>MSKKRVVKLRELVPAVAALAVAVLIQSATGSSGGSGHTPTTQATHADDHDLTTHNGTEEHDDGHDDGHDDLHAHAPKVIVFISGSCLFGAISRSLFKKLPIPYTVVLLILGAILGVVASNVPLVEEHTRDVAHMDPHVLLQIFLPVLIFESAFAMDVHTFMRSFSQVCILALFGLVVASVLTAVLAMNLFNYNWNFSEAMMFGAIMSATDPVAVVALLKDLGASKQLGTIIEGESLLNDGCAIVIFNVFMKMVFFPQLTSTVGQNVLYFLQVAVAGPLWGYAVAKVTVFFLSHIFNDALVEITITLAATYLTYYIGDIWLEVSGVLAVVVLGLIVNAEKTSISPEVEVFLHRFWEMLAYLANTLIFMMVGVVVTQKALVAVDKMDWFYLIILYLAIT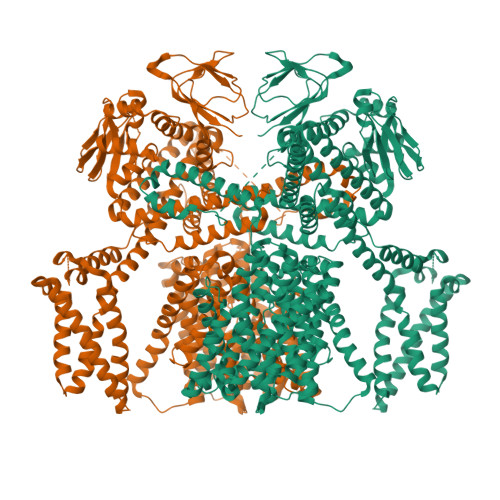IIRGMVISLFSPILSRIGYGLTWRNAVIMTWGGLRGAVGLALALVVENLAGNDVIGSKFLFHTAGIVVLTLVINATTIQTLLRILGMSDISIPKRLAMAGAVRRIHEGQNRTLNMLKSDRFLADADWDIATAACEISDPYSALSDDENAPADELTLGERKSVCPGCKAMVPNEPSPREFADMMEEARLRMLKAEKISYWKQFEHGMLAREALRLLVQHAEVAADEKDQFILVDDLKKSWQIKGIYPWLKRKLEDLISEKKIAAIPMPKYKLGKLMYKICHHMAFEVTINIAIVLNIVPIIMEFVVQDKMASVSTMAAPGSTVSSEPSSLQKIEDALRISNYVFFVIYAIEAIVKILGLGRHYIVSHWNKFDAFILVVALVDIIIAETLLKGSITINLSSIKVVKLFRLLRGLRMLRLTKALIPKLILVVNGKINNQLSLGYDVGKGYIIGEEEVGKIIDRMVDNKKILRELKHISETGRLQVVKELGLLQREHPGIAVSVKTRQAIRTILNHSRETIHELQGAGLLDEMEAHKLELTVEIKMKRLMNAPSSIPPPPPENLLKNVSWLAGDMKLIDFIKARASLLHFDYGEVIVREGDESDGLFLIVSGLVKLYGKSAFLDHDNPPVTAGSEENEVFEDYLTVGNVIGEMGVLTKKPRNATVTCETTVQVYFITAEDMNIAIDTFTLYPSLEYRLWRVVAIRIATPLIMEQMAFQGWTQEKVKLHLERGYLVDLAESHFQFNIDATLEDVILINGTAYNAHTREEIRSPCLISRTVHKLTFQYTATEEPRLFVVRNAEYNGPILDGRLDVDSKRSLISITEISSNMCLKHAAELRQKNSKVMLSRKSSGAAAKEEEDCIPNTSDVEQAAGVSPSVPTKTTPKPKSFLPSLGLSMSKERVNGEAVEESPVKTKQGEETPETEEGAAPRVNVALEVLFQ[2x]>[2x]MSLHYQPKQDLLNDRIILVTGASDGIGREA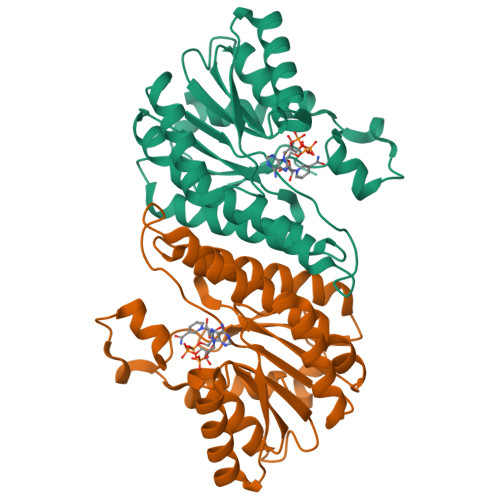AMTYARYGATVILLGRNEEKLRQVASHINEETGRQPQWFILDLLTCTSEDCQQLAQRIAVNYPRLDGVLHNAGLLGDVCPMSEQDPQVWQDVMQVNVNATFMLTQALLPLLLKSDAGSLVFTSSSVGRQGRANWGAYAASKFATEGMMQVLADEYQQRLRVNCINPGGTRTAMRASAFPTEDPQKLKTPADIMPLYLWLMGDDSRRKTGMTFDAQPGRKPGISQEGHHHHHH>MGQGPELHLASQFVNEACRALVFGGCVEKSSVSRNPEVPFESSAYRISASARGKELRLILSPLPGAQPQQEPLALVFRFGMSGSFQLVPREELPRHAHLRFYTAPPGPRLALCFVDIRRFGRWDLGGKWQPGRGPCVLQEYQQFRENVLRNLADKAFDRPICEALLDQRFFNGIGNYLR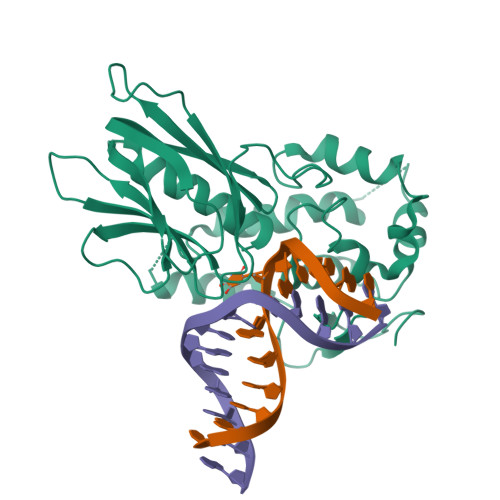AEILYRLKIPPFEKARSVLEALQQHRPSPELTLSQKIRTKLQNPDLLELCHSVPKEVVQLGGKGYGSESGEEDFAAFRAWLRCYGMPGMSSLQDRHGRTIWFQGDPGPLAPKGRKS[3x]4-AMINO-6-CHLOROBENZENE-1,3-DISULFONAMIDE 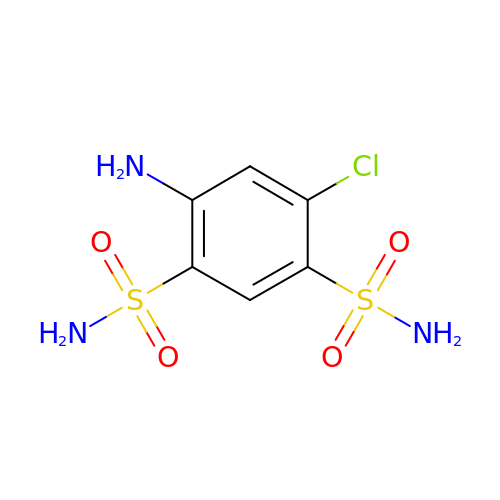| C6 H8 Cl N3 O4 S2 | IHJCXVZDYSXXFT-UHFFFAOYSA-N A similar mechanism underlying channel activation also applies to the ion channel TMEM16A, which opens in response to an increase in the intracellular Ca2+ concentration (Caputo et al, 2008; Schroeder et al, 2008; Yang et al, 2008). TMEM16A mediates important physiological processes such as epithelial chloride transport and smooth muscle contraction and has been proposed to be a therapeutic target for diseases including asthma, hypertension, stroke, and cystic fibrosis (Huang et al, 2012; Danahay et al, 2020; Al‐Hosni et al, 2022; Galietta, 2022). The protein is a homodimer, with each subunit containing an ion conduction pore and a principal Ca2+‐binding site that are closely apposed (Dang et al, 2017; Paulino et al, 2017a, 2017b). Both pores act independently and are activated by the binding of two Ca2+ ions to the principal site (Jeng et al, 2016; Lim et al, 2016).

In addition to this ionic interaction, our previous study has identified several residues around the Ca2+‐binding site as important determinants of channel activation, which is manifested by a profound decrease in the potency of Ca2+ upon mutation to alanine (Lam et al, 2021). Here, we focus on Leu 647 on α6 and Ile 733 on α8, both within the π‐helical region, which are brought into van der Waals contact in the Ca2+‐bound state upon α6 activation (Figs 1 and EV1). To understand the rearrangements underlying the efficacy of pore opening, we determined a cryo‐EM structure of L647V/I733V, whose gating properties are similarly affected compared to the less conservative mutant L647A/I733A but which is characterized by a more severely perturbed ion conduction pathway, in the presence of a saturating Ca2+ concentration (and Fig EV2). With an overall resolution of 3.29 Å, the final map shows well‐defined density for the entire protein, including the bound agonist Ca2+ in its principal binding site (Fig EV2G and H). Single‐particle analysis of L647V/I733V reveals a major conformation that is distinct from the wild‐type channel (Fig EV2). In this structure, the disruption of the L647/I733 interaction results in an incomplete rearrangement of α6, with the helix adopting an intermediate, partially activated conformation. The described change in conformation is accompanied by a loss of the density corresponding to the Ca2+‐binding part of α6, indicating that the helix has become more mobile and that the interaction with bound Ca2+ is substantially weakened (Fig EV2G and H). The single‐bound Ca2+ is in a position similar to the lower ion in the doubly bound state and is coordinated by two acidic residues, Glu 705 on α7 and Asp 738 on α8, with no coordinating residues from α6 since its rearrangement is impaired.

>[2x]MRVPEKYSTLPAEDRSVHIVNICAIEDLGYLPSEGTLLNSLSVDPDAECKYGLYFRDGKRKVDYILVYHHKRASGSRTLARRGLQNDMVLGTRSVRQDQPLPGKGSPVDAGSPEVPMDYHEDDKRFRREEYEGNLLEAGLELENDEDTKIHGVGFVKIHAPWHVLCREAEFLKLKMPTKKVYHISETRGLLKTINSVLQKITDPIQPKVAEHRPQTTKRLSYPFSREKQHLFDLTDRDSFFDSKTRSTIVYEILKRTTCTKAKYSMGITSLLANGVYSAAYPLHDGDYEGDNVEFNDRKLLYEEWASYGVFYKYQPIDLVRKYFGEKVGLYFAWLGAYTQMLIPASIVGVIVFLYGCATVDENIPSMEMCDQRYNITMCPLCDKTCSYWKMSSACATARASHLFDNPATVFFSVFMALWAATFMEHWKRKQMRLNYRWDLTGFEEEEEAVKDHPRAEYEARVLEKSLRKESRNKETDKVKLTWRDRFPAYFTNLVSIIFMIAVTFAIVLGVIIYRISTAAALAMNSSPSVRSNIRVTVTATAVIINLVVIILLDEVYGCIARWLTKIEVPKTEKSFEERLTFKAFLLKFVNSYTPIFYVAFFKGRFVGRPGDYVYIFRSFRMEECAPGGCLMELCIQLSIIMLGKQVIQNNLFEIGIPKMKKFIRYLKLRRQSPSDREEYVKRKQRYEVDFNLEPFAGLTPEYMEMIIQFGFVTLFVASFPLAPLFALLNNIVEIRLDAKKFVTELRRPVAIRAKDIGIWYNILRGVGKLAVIINAFVISFTSDFIPRLVYLYMYSQNGTMHGFVNHTLSSFNVSDFQNGTAPNDPLDLGYEVQICRYKDYREPPWSEHKYDISKDFWAVLAARLAFVIVFQNLVMFMSDFVDWVIPDIPKDISQQIHKEKVLMVELFMREEQGKQQLLDTWMEKEKPRDVPCNNHSPTTHPEAGDGSPVPSYEYHGDAL>[6x]SNAMEVTDVRLRRVNTDGRMRAIASITLDHEFVVHDIRVIDGNNGLF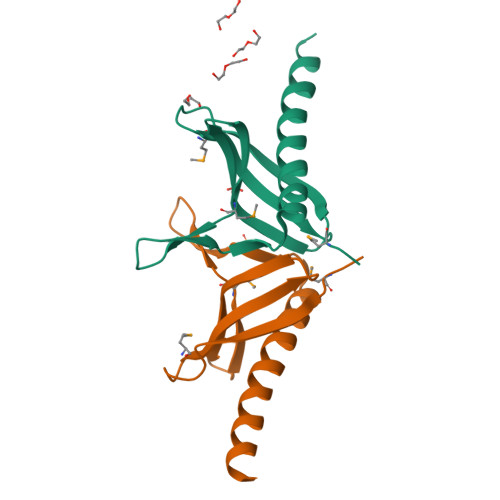VAMPSKRTPDGEFRDITHPINSSTRGKIQDAVLNEYHRLGDTEALEFEEAGAS>[2x]ADLLVKTPEAYDQALKKAKPGDDIILANGTWRDFEVLFEAKGNENKPITLRGQTPGKVFLTGQSNLRLAGEHLIVSGLVFKDGYTPTGEVIAFRRNKDVLASHSRVTQVVIDNFSNPEKFEQDSWVMVYGRHNRFDHNHLVGKRNKGVTMAVRLTTESSQQNHHRIDHNYFGPRPILGSNGGETLRIGTSHHSLTDSFTLVENNYFDRCNGEVEIISNKSGKNSIRNNVFFESRGTLTLAHGNGNIVENNVFFGNGVDHTGGIRVINRDQIIRNNYLEGLTGYRFGSGLTVMNGVPNSKINRYHQVDNALIENNTLVNVEHIQFAAGSDKERSAAP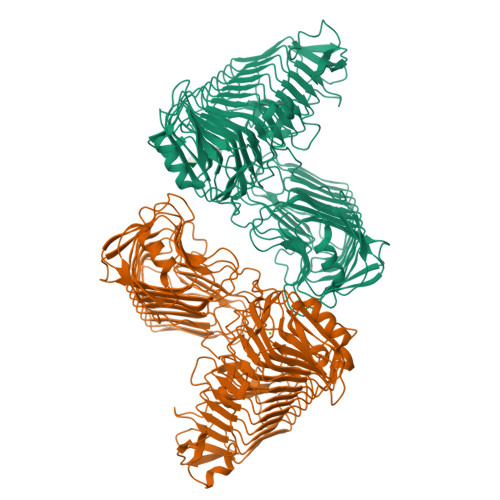INSNMNNNLIVNDQGTDGITAFDDISGIKFKDNLLNQDAKPSINKGFEQADITMQRHDNGLLYPEAKTQQKYGVSTQLEPIGKDEVGVSWYPKVEPDVAFGSGKHIAVSPGDNTLFDAIASAETGDVLVLQAGEYWVSKILSLDKTLTIRAQEKGSAVIFPQRSTLIEINNKGNLTLDGVYVDATNAPDAAGNTLIRTTRLPMQRNYRLAIKNSTFENLDINHSYHFFDAGNRSFADYIEVQDSQFKHITGDLFRLNKETDDLGIYNVEYLTIENSNVSDLQGAIAKVYRGGTDESTFGPHVVMNNNIFNEVGKGKRNKSAASLILHGTQVNKMTTNEFNNSAPIIFELTVGEPKTWVTGNVFEGTPEPVVRDLFPLSGATTTISGNTVL High-potential iron-sulfur protein (HiPIP) is a small (~10 kDa) soluble protein functioning as an electron carrier in photosynthetic Gram-negative bacteria. HiPIP supplies an electron from the cytochrome bc1 complex to the photosynthetic reaction center (RC) in order to re-reduce a special pair of chlorophyll molecules in the RC. The protein possesses one Fe4S4 cluster at the molecular center. The cluster changes its redox state between [Fe4S4]2+ and [Fe4S4]3+.

Here, we report the preparation and X-ray crystallographic analysis of the oxidized HiPIP at 0.8 Å resolution. The oxidized form of HiPIP was prepared by treatment with the oxidizing agent K3[Fe(CN)6]. Therefore, crystals of the oxidized state were produced from the oxidized HiPIP in the solution in order to elucidate the true structural differences accompanying the redox changes. The refined structure of the oxidized HiPIP contains all 83 residues, one Fe4S4 cluster, three glycerols, five sulfate ions and 160 water molecules. No ferricyanide ions are observed in the electron density map. The intra-subcluster bond lengths are decreased by the oxidation, while inter-subcluster bond lengths are not. The largest changes are observed in the Fe−S bonds around Fe1 and Fe2. In addition, the bond lengths of Fe- (Cys-Sγ) for all Fe atoms are also decreased by the oxidation. Our results for the difference in the Fe-S lengths implies that the subcluster composed of Fe1, Fe2, S3, and S4 is important for storing electronic charges in HiPIP. In addition, most distances between the sulfur atoms of the iron-sulfur cluster and the protein environment are elongated upon the oxidation.

> AAPANAVTADDPTAIALKYNQDATKSERVAAARPGLPPEEQHCANCQFMQANVGEGDWKGCQLFPGKLINVNGWCASWTLKAG> GKDNTKVIAH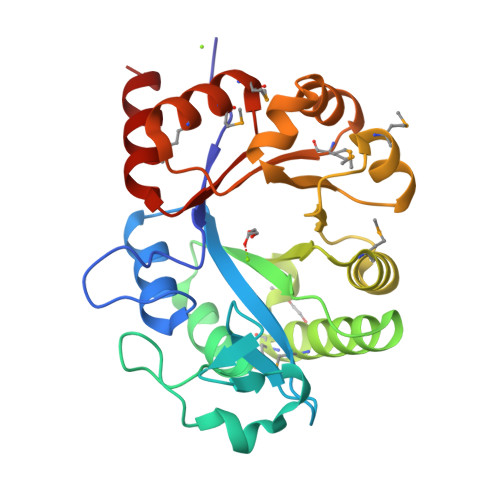RGYWKTEGSAQNSIRSLERASEIGAYGSEFDVHLTADNVLVVYHDNDIQGKHIQSCTYDELKDLQLSNGEKLPTLEQYLKRAKKLKNIRLIFELKSHDTPERNRDAARLSVQMVKRMKLAKRTDYISFNMDACKEFIRLCPKSEVSYLNGELSPMELKELGFTGLDYHYKVLQSHPDWVKDCKVLGMTSNVWTVDDPKLMEEMIDMGVDFITTDLPEETQKILHSRAQ>GSAMGQNPWATTTAFADFMKRFNIPQVHGSGIFVDLGRDTEGYREVGGKCPVFGKAIQMHQPAEYSNNFLDDAPTSNDASKKPLPGGFNNPQVYTSGQKFSPIDDSLLQERLGTAGPKTAIGRCALYAYSTIAVNPSTNYTSTYKYPFVYDAVSRKCYVLSVSAQLLKGEKYCSVNGTPSGLTWACFEPVKEKSSARALVYGSAFVAEGNPDAWQSACPNDAVKDALFGKWEDGQCVPFDTKTSVQSDQATNKEECWKRVFANPLVASDAPTTYPEAAQKNWNDFWPVHEQSSPKSGGFGANWANFYLEKESGETICAIFDQVPDCFAPITGAVAYTALGSSTEVNLPQCDSASFIPIEGPCNNCVQVVT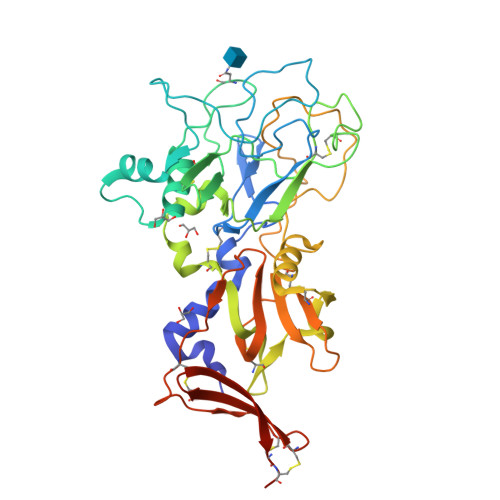ECVGNQFDQTSKACCTEPEAAALVPR[12x]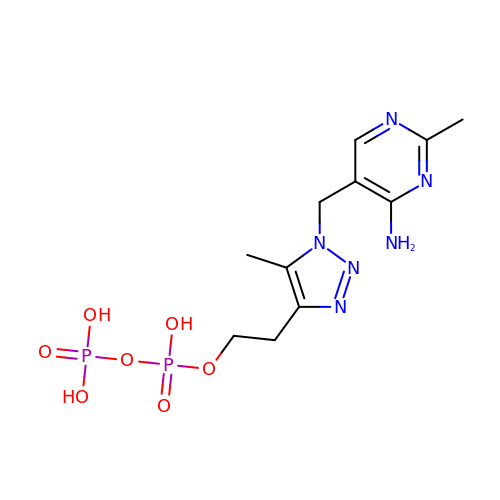2-{1-[(4-AMINO-2-METHYLPYRIMIDIN-5-YL)METHYL]-5-METHYL-1H-1,2,3-TRIAZOL-4-YL}ETHYL TRIHYDROGEN DIPHOSPHATE | C11 H18 N6 O7 P2 | WHMXQEYVWLIXHH-UHFFFAOYSA-N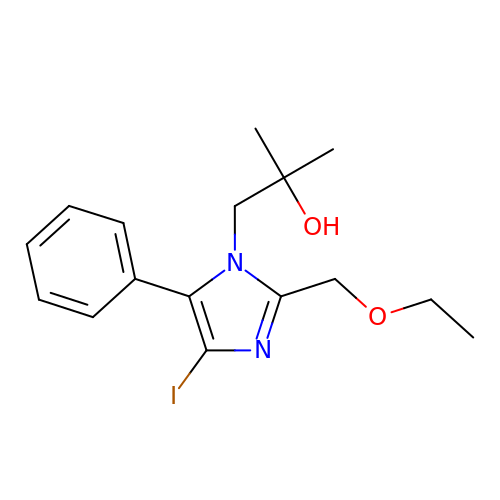1-[2-(ethoxymethyl)-4-iodanyl-5-phenyl-imidazol-1-yl]-2-methyl-propan-2-ol | C16 H21 I N2 O2 | XCYMSVIYUJTAPJ-UHFFFAOYSA-N> MKETNFGEKTRVLVVGGTGSLGRRIVSACLAEGHETYVLQRPEIGVDIEKVQLLLSFKRLGAHLVEGSFSDHQSLVSAVKQVDVVVSAMSGVHFRTHNI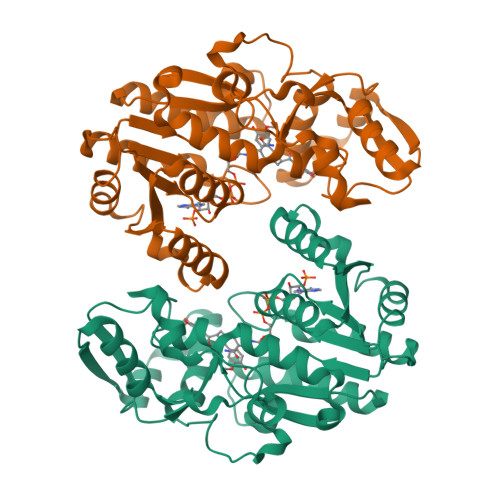PVQLKLVAAIKEAGNVKRFLPSEFGMDPSRMGHAMPPGSETFDQKMEIRNAIKAAGISHTYLVGACFAAYFGGNLSQMGTLFPPKNKVDIYGDGNVKVVFVDEDDMAKYTAKTLNDPRTLNKTVYVRPTDNILTQMELVQIWEKLTEKELEKTYVSGNDFLADIEDKEISHQAGLGHFYHIYYEGCLTDHEVGDDEEATKLYPDVKYKRMDEYLKIFV>MAVDADSANYRIEHDTMGEVRVPAKALWRAQTQRAVENFPISGRGLERTQIRALGLLKGACAQVNSDLGLLAPEKADAIIAAAAEIADGQHDDQFPIDVFQTGSGTSSNMNTNEVIASIAAKGGVTLHPNDDVNMSQSSNDTFPTATHIAATEAAVAHLIPALQQLHDALAAKALDWHTVVKSGRTHLMDAVPVTLGQEFSGYARQIEAGIERVRACLPRLGELAIGGTAVGTGLNAPDDFGVRVVAVLVAQTGLSELRTAANSFEAQAARDGLVEASGALRTIAVSLTKIANDIRWMGSGPLTGLAEIQLPDLQPGSSIMPGKVNP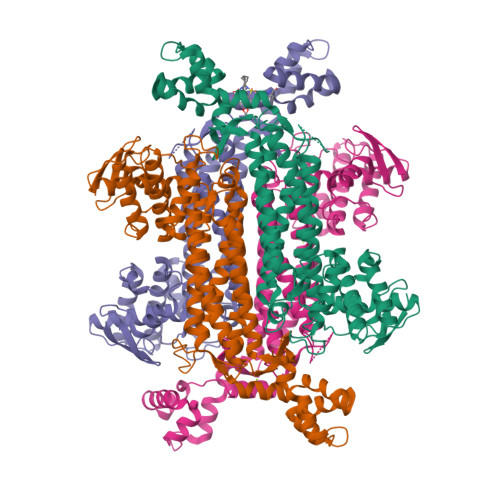VLPEAVTQVAAQVIGNDAAIAWGGANGAFELNVYIPMMARNILESFKLLTNVSRLFAQRCIAGLTANVEHLRRLAESSPSIVTPLNSAIGYEEAAAVAKQALKERKTIRQTVIDRGLIGDRLSIEDLDRRLDVLAMAKAEQLDSDRL[4x]>[2x]MRSRRVDVMDVMNRLI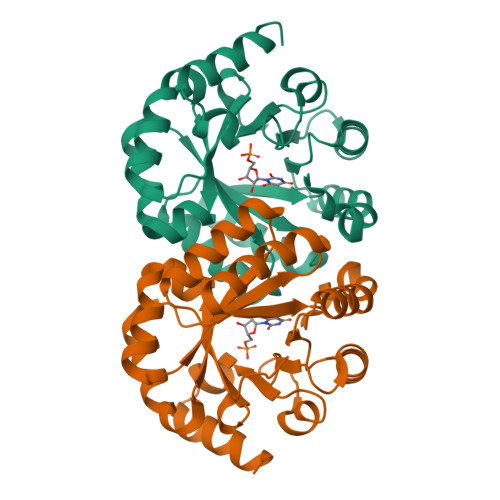LAMDLMNRDDALRVTGEVREYIDTVKIGYPLVLSEGMDIIAEFRKRFGCRIIADFKVADIPETNEKICRATFKAGADAIIVHGFPGADSVRACLNVAEEMGREVFLLTEMSHPGAEMFIQGAADEIARMGVDLGVKNYVGPSTAPERLSRLREIIGQDSFLISPGVGAQGGDPGETLRFADAIIVGASIYLADNPAAAAAGIIESIKDLLNP> MSGGDRFVQTLQKLNYPKGAQLDGEDFDWLFEAVDLKPFLDWFCSAASEQNVVPDEKLQAFNTLKESGKPVLDEKALDEVLKTFSISKVPAIEEVAIEKLEEEVKALQKQKNLHIRRRNKLQMVESGNRQMCLKSKDKEEETGRAFQEVLHLLRVTNKKLNHELQSIV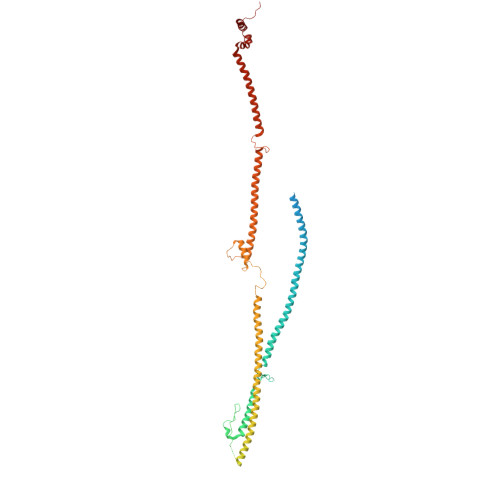NGVQTLMSFFSTPETACELSSQPIFLSQLLLDKYLSLEEQSTAALTSFTKEHFFEGMSKFVEGSDENFQLVQLNVNSFGEDGTTEDKCKEMMRLQLAYICAKHKLIQMKAKSASLKVGLQWAENNASVVQDKASQKEENLKVRITSLKNETLQIENHTNSISNEKLPGLVRDNAQLLNMPIVKGDYDLQMAHQTSCSSRQDLVCDHLMKQKASFELLQLGYELELRKHRDVYRELGSIVQELKESGDKLEERLTMLSDVNLLSASKPRSNIDSKDLTSHRLYQLLDGDNTQKLFRTYDGLESVAQKLSQDIASMRDQLEVSEQEHSLLLSKLDSHLKELRDFMYPEGNTLMLTTPELSGEFHQLGSQLEKLNHITVEILGDLQLKRKMLESNKLQQIEKQLYVYFFQNEEQLKSIVGKLEAQTGGGSSA>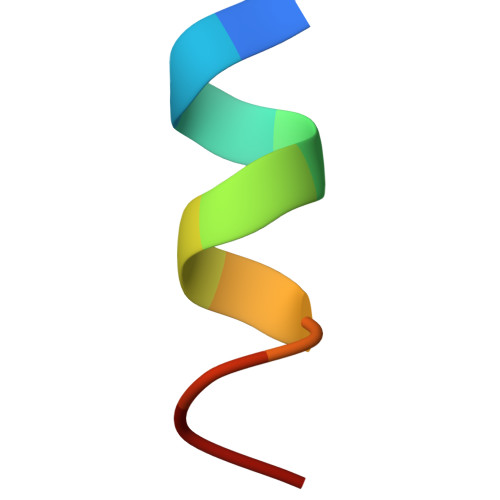 PALTAVETGAT> VLQLKL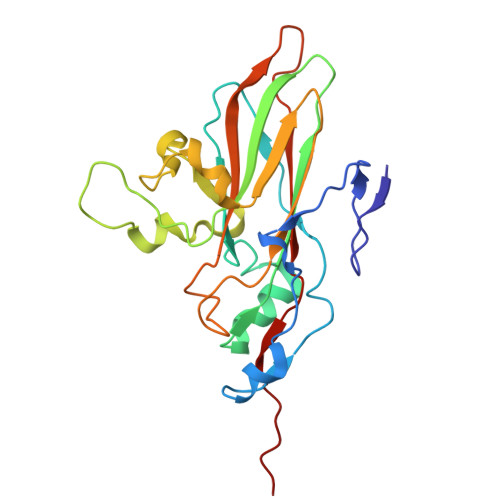GNSAIVTQEAANMCCAYGEWPSYLPDNEATAIDKPTQPETSTDRFYTLKSVKWEGTSTGWWWKLPDALNQTGMFGQNVQYHYLYRSGFLCHVQCNATKFHQGALLVVAIPEHQLGKYNTGTSASFDDVMKGKTGGVFTHPYVLDDGTSLACSLIFPHQWINLRTNNSATIMLPWMNCAPMDFALRHNQWTLAIIPVVPLNTSGGTTMVPITVSIAPMCCEFNGLRNAITQ>GTVFRQENVDDYYDTGEELGSGQFAVVKKCREKSTGLQYAAKFIKKRRTKSSRRGVSREDIEREVSILKEIQHPNVITLHEVYENKTDVILILELVAGGELFDFLAEKESLTEEEATEFLKQILNGVYYLHSLQIAHFDLKPENIMLLDRNVPKPRIKIIDFGLAHKIDFGNEFKNIFGTPEFVAPEIVNYEPLGLEADMWSIGVITYILLSGASPFLGDTKQETLANVSAVNYEFEDEYFSNTSALAKDFIRRLLVKDPKKRMTIQDSLQHPWIKPK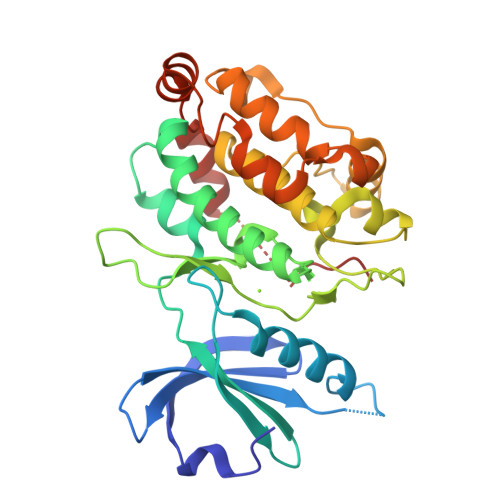DTQQALSRKASAVNMEKFKKFAARKKWKQSVRLI[2x]> RSRRVDVMDVMNRLILAMDLMNRDDALRVTGEVREYIDTVKIGYPLVLSEGMDIIAEFRKRFGCRIIADFKVADIPETNEKICRATFKAGADAIIVHGFPGADSVRACLNVAEEMGREVFLLTEMSHPGAEMFIQGAADEIARMGVDLGVKNYVGPSTRPERLSRLREIIGQDSFLISPGVGAQGGDPGETLRFADAIIVGRSIYLAD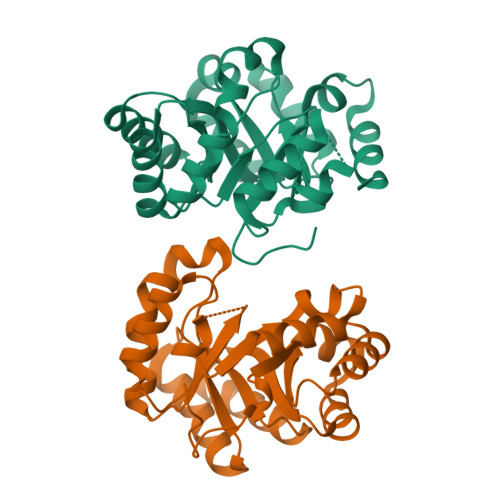NPAAAAAGIIESIKDLLNP>[6x]MSKSVFVGELTWKEYEARVAAGDCVLMLPVGALEQHGHHMCMNVDVLLPTAVCKRVAERIGALVMPGLQYGYKSQQKSGGGNHFPGTTSLDGATLTGTVQDII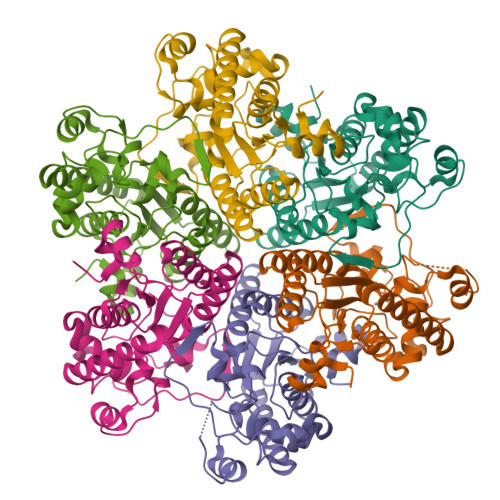RELARHGARRLVLMNGHYENSMFIVEGIDLALRELRYAGIQDFKVVVLSYFDFVKDPAVIQQLYPEGFLGWDIEHGGVFETSLMLALYPDLVDLDRVVDHPPATFPPYDVFPVDPARTPAPGTLSSAKTASREKGELILEVCVQGIADAIREEFPPT>MGSDKIHHHHHHMSLRDKIEELKKIEKEIEQGGGPEKVEKQHRAGKLTAWERLELLLDPGTFVEIDKFVEHRNTYFGLDKVKLPRDGVITGVGEINGRKVAVFSQDFTVMGGSLGEMHAKKIVKLLDLALKMGIPVIGINDSGGARIQEGVDALAGYGEIFLRNTLASGVVPQITVIAGPCAGGAVYSPALTDFIVMVDQTARMFITGPNVIKAVTGEEISQEDLG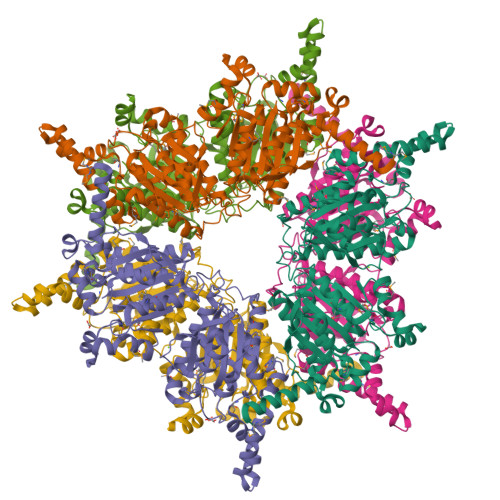GAMVHNQKSGNAHFLADNDEKAMSLVRTLLSYLPSNNAEEPPVEDPDTSLETPEDILDILPDNPNKGYDVRDVIKRVVDHGEFFEVQPYFAKNIVIGFARIQGKTVGIVANQPSVLAGVLDIDSSDKAARFIRFLDAFNIPILTFVDTPGYLPGVAQEHGGIIRHGAKLLYAYSEATVPKITVILRKAYGGAYIAMGSKHLGADMVLAWPSAEIAVMGPEGAANIIFKREIEASSNPEETRRKLIEEYKQQFANPYIAASRGYVDMVIDPRETRKYIMRALEVCETKVEYRPKKKHGNIPL[6x]>SMKLTIPELSLVVLIGSSGSGKSTFAKKHFKPTEVISSDFCRGLMSDDENDQTVTGAAFDVLHYIVSKRLQLGKLTVVDATNVQESARKPLIEMAKDYHCFPVAVVFNLPEKVCQERNKNRTDRQVEEYVIRKHTQQMKKSIKGLQREGFRYVYILN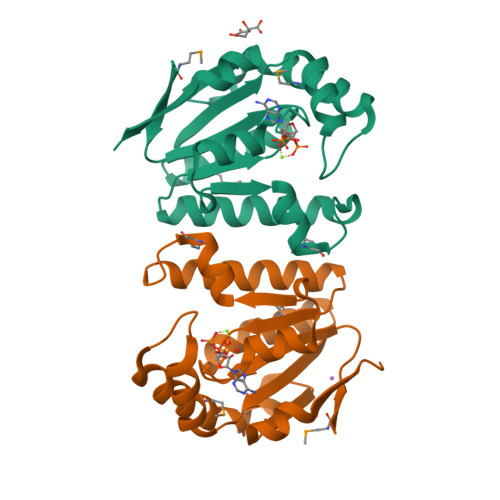SPEEVEEVVFERQP[2x]>[2x]AECSVDIQGNDQMQFNTNAITVDKSC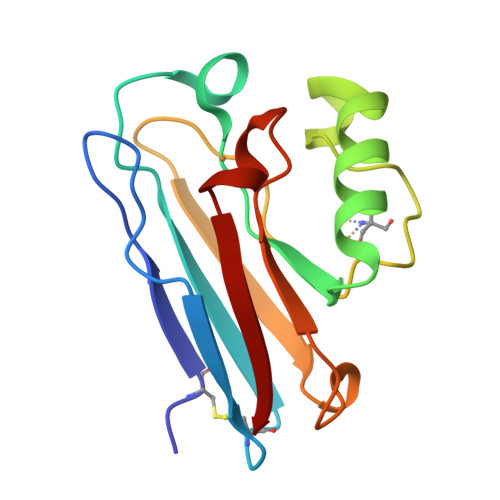KQFTVNLSHPGNLPKNVMGENWVLSTAADMQGVVTDGMASGLDKDYLKPDDSRVIAHTKLIGSGEKDSVTFDVSKLKEGEQYMFFCTFPGHSALHKGTLTLK(2~{S})-2-azanyl-4-[[(2~{S},3~{S},4~{R},5~{R})-5-[4-azanyl-5-[2-(1~{H}-benzimidazol-2-yl)ethynyl]pyrrolo[2,3-d]pyrimidin-7-yl]-3,4-bis(oxidanyl)oxolan-2-yl]methylsulfanyl]butanoic acid | C24 H25 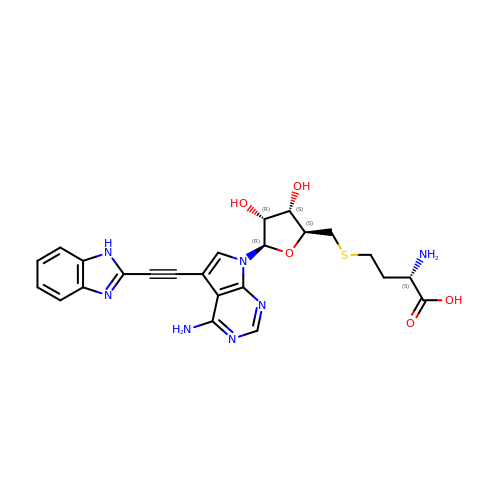N7 O5 S | PYEFDSOFRINBSR-IMYLTZEYSA-N>[4x]VEQELATKMLQIQSKRFYLDVKQNRRGRFIKVAEIGADG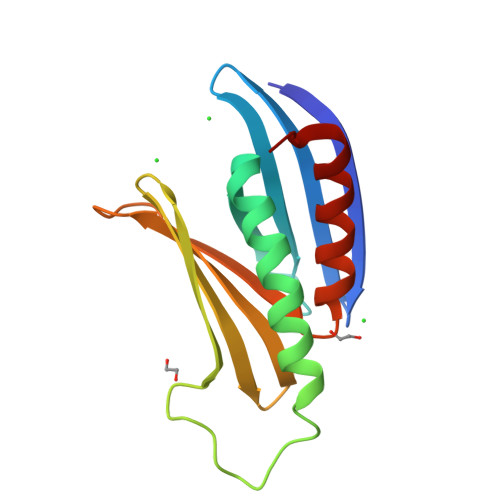RRSQIYLALSTAAEFRDHLSSFSDYYASLGPPNTDNLPEDGKLKSEMMIKDYRRYYLDLKENARGRFLRVSQTITRGGPRSQIALPAQGMIEFRDALTDLLEEFGAN Although amyloid fibers and oligomers of two proteins, tau and amyloid-β, have been identified in association with this disease, the development of diagnostics and therapeutics has proceeded to date in a near vacuum of information about their structures. Here we report the first atomic structures of small molecules bound to amyloid. These are of the dye orange-G, the natural compound curcumin, and the Alzheimer's diagnostic compound DDNP bound to amyloid-like segments of tau and amyloid-β. Negatively charged orange-G wedges into a specific binding site between two sheets of the fiber, combining apolar binding with electrostatic interactions, whereas uncharged compounds slide along the cavity. The amyloid components in our structures are steric zippers formed by stacks of six-residue segments from Alzheimer-related proteins.

The VQIVYK segment of tau was suggested as the minimal interaction motif for fiber formation. We previously determined the crystal structure of VQIVYK in two crystal forms; both show the common steric zipper motif of amyloid fiber-like structures. Co-crystallization of VQIVYK with orange-G resulted in deep orange crystals. Mass spectrometric analyses of the crystals showed relatively high abundance of orange-G (∼1∶10 molar stoichiometry with VQIVYK). Determination of the structure revealed a new crystal form of VQIVYK. Similar to Form-1, the steric zipper shows a tight and dry interface; yet there is a large void between pairs of steric zipper, in contrast to the tightly packed structure of Form-1. Orange-G is situated within this void, binding between lysine side chains facing each other from two parallel pairs of zippers, forming an electrostatic network that also involves zinc cations. As in its complex with KLVFFA, orange-G lies with its long axis parallel to the fiber axis. In the complex with VQIVYK, the aromatic rings of orange-G are also packed against apolar side chains, but the binding is largely mediated via polar interactions with glutamine and lysine side-chains at the edges of two steric zippers. Crystallization of VQIVYK alone, under identical conditions to the co-crystallization of the VQIVYK-orange-G mixture, resulted in the formation of colorless fibrous crystals giving poor X-ray diffraction.

> VQIVYK>[2x]SDKIIHLTDDSFETDVLKADGAILVDFWAEWCGPCKMIAPILDEIADEYQGKLTVA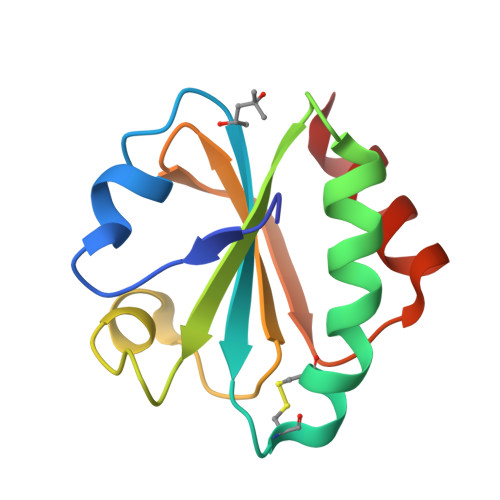KLNIDQNPGTAPKYGIRGIPTLLLFKNGEVAATKVGALSKGQLKEFLDANLA>ADPGAPAPVNPCCYYPCQHQGICVRFGLDRYQCDCTRTGYSGPNCTIPEIWTWLRTTLRPSPSFIHFLLTHGRWLWDFVNATFIRDTLMRLVLTVRSNLIPSPPTYNIAHDYISWESFSNVSYYTRILPSVPRDCPTPMGTKGKKQLPDAEFLSRRFLLRRKFIPDPQGTNLMFAFFAQHFTHQFFKTSGKMGPGFTKALGHGVDLGHIYGDNLERQYQLRLFKDGKLKYQMLNGEVYPPSVEEAPVLMHYPRGIPPQSQMAVGQEVFGLLPGLMLYATIWLREHNRVCDLLKAEHPTWGDEQLFQTARLILIGETIKIVIEEYVQQLSGYFLQLKFDPELLFGAQFQYRNRIAMEFNQLYHWHPLMPDSFRVGPQDYSYEQFLFNTSMLVDYGVEALVDAFSRQPAGRIGGGRNIDHHILHVA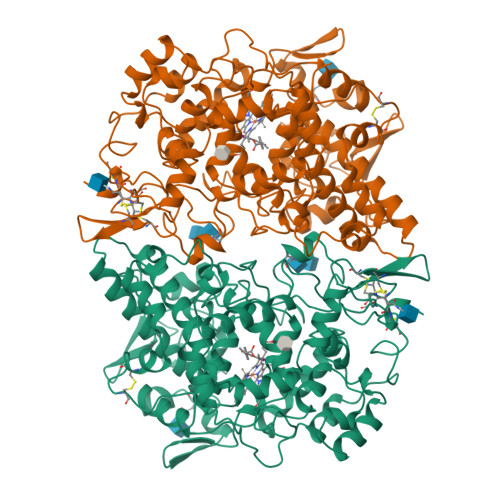VDVIKESRVLRLQPFNEYRKRFGMKPYTSFQELTGEKEMAAELEELYGDIDALEFYPGLLLEKCHPNSIFGESMIEMGAPFSLKGLLGNPICSPEYWKASTFGGEVGFNLVKTATLKKLVCLNTKTCPYVSFHVPDPRQEDRPGVERPPTEL[2x]>[2x]MKFPKDFMIGYSSSPFQFEAGIPGSEDPNSDWWVWVHDPENTAAGLVSGDFPENGPGYWNLNQNDHDLAEKLGVNTIRVGVEWSRIFPKPTFNVKVPVERDENGSIVHVDVDDKAVERLDELANKEAVNHYVEMYKDWVERGRKLILNLYHWPLPLWLHNPIMVRRMGPDRAPSGWLNEESVVEFAKYAAYIAW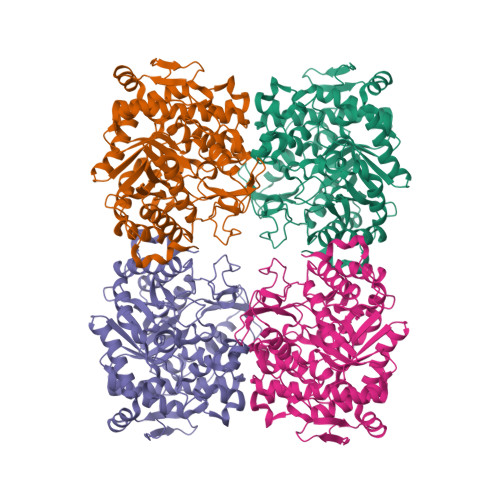KMGELPVMWSTMNEPNVVYEQGYMFVKGGFPPGYLSLEAADKARRNMIQAHARAYDNIKRFSKKPVGLIYAFQWFELLEGPAEVFDKFKSSKLYYFTDIVSKGSSIINVEYRRDLANRLDWLGVNYYSRLVYKIVDDKPIILHGYGFLCTPGGISPAENPCSDFGWEVYPEGLYLLLKELYNRYGVDLIVTENGVSDSRDALRPAYLVSHVYSVWKAANEGIPVKGYLHWSLTDNYEWAQGFRQKFGLVMVDFKTKKRYLRPSALVFREIATHNGIPDELQHLTLIQ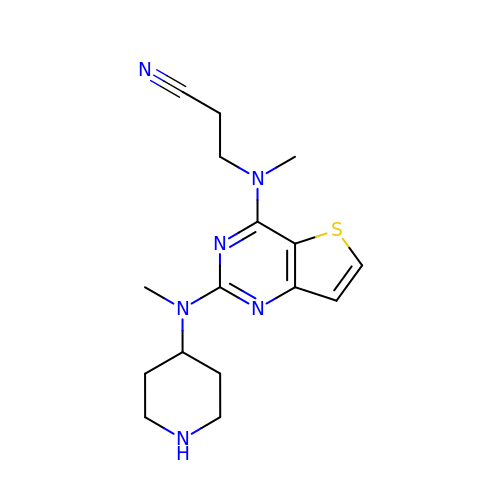3-[methyl-[2-[methyl(piperidin-4-yl)amino]thieno[3,2-d]pyrimidin-4-yl]amino]propanenitrile | C16 H22 N6 S | ZZVMFUZVPCVUGH-UHFFFAOYSA-N>[2x]HQYLLPEAKAQDSDKICVVINLDETLVHSSFKPVNNADFIIPVEIDGVVHQVYVLKRPHVDEFLQRMGELFECVLFTASLAKYADP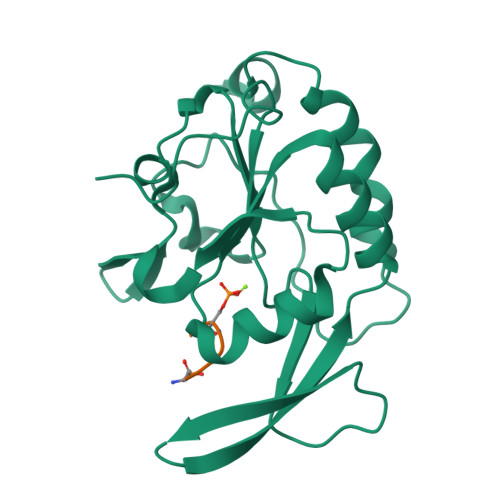VADLLDKWGAFRARLFRESCVFHRGNYVKDLSRLGRDLRRVLILDNSPASYVFHPDNAVPVASWFDNMSDTELHDLLPFFEQLSRVDDVYSVLRQ;>PSYSPTSPS[2x]> ANSGEAPKNFGLDVKITGESENDRDLGTAPGGTLNDIGIDLRPWAFGQWGDWSAYFMGQAVAATDTIETDTLQSDTDDGNNSRNDGREPDKSYLAAREFWVDYAGLTAYPGEHLRFGRQRLREDSGQWQDTNIEALNWSFETTLLNAHAGVAQRFSEYRTDLDELAPEDKDRTHVFGDISTQWAPHHRIGVRIHHADD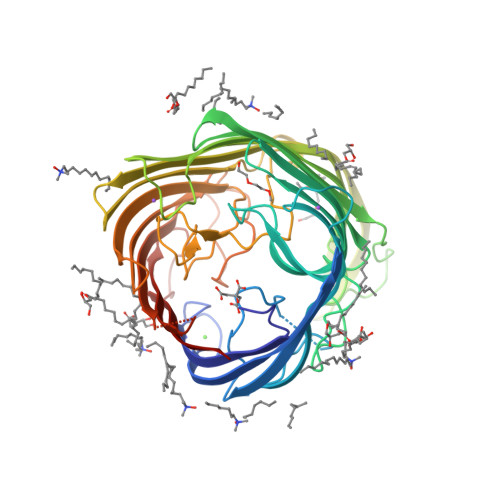SGHLRRPGEEVDNLDKTYTGQLTWLGIEATGDAYNYRSSMPLNYWASATWLTGDRDNLTTTTVDDRRIATGKQSGDVNAFGVDLGLRWNIDEQWKAGVGYARGSGGGKDGEEQFQQTGLESNRSNFTGTRSRVHRFGEAFRGELSNLQAATLFGSWQLREDYDASLVYHKFWRVDDDSDIGTSGINAALQPGEKDIGQELDLVVTKYFKQGLLPASMSQYVDEPSALIRFRGGLFKPGDAYGPGTDSTMHRAFVDFIWRF>[2x]MSLKYIIGMDVGTTATKGVLYDINGKAVASVSKGYPLIQTKVGQAEEDPKLIFDAVQEIIFDLTQKIDGKIAAIS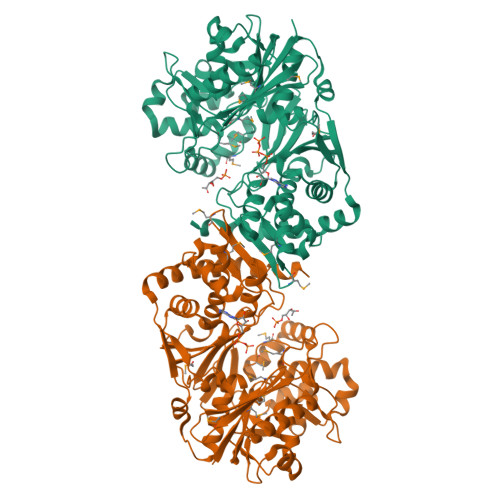WSSQMHSLIGLGSDDELLTNSITWADNCAKSIVQDAKNRGFAQQIYRKTGMPMHPMAPIYKLLWLKNKKTEVFSQAQKWIGIKEYIIFRLTGKLVTDTTMAAGTGILNLKTLTWDQELLDILKIKKEQLPKIAQPTKVIFPIKTEYVKKLGIDSDTKIILGASDGYLSTIGVNAIDSDHCALNVGTSGAIRTIVDQPKIDPSASYFCYPADKTHYLLGGPVNNGGIVFNWARQTLFDADETPQDFLDVAQTAPAGSRNLIFLPYLGGERAPIWDANARGSFVGLTRMHQKPEMARAVIEGIIFNLYDAASNLIKNTKKPVAINATGGFLKSDFVRQLCANIFNVPIVTMKEQQSGTLAAMFLARQALGLNQDLSEIGQFAQADKVYFPNPKEAATYQKLFPLYCEIRNALAASYGKFSNINEGHHHHHH>MNIIAILNHMGVYFKEEPIRELHKALEALDFQIVYPNDREDLLKLIDNNARLCGVIFDWDTYNLDLCEEISAMNEHLPVYAFANTHSTLDVSLNDLRLNVEFFEYALGAAQDIAQKIRQSTDAYIDEILPPLTKALFNYVKEGKYTFCTPGHMGGTAFQKSPVGSIFYDFFGANAMKSDISISVGELGSLLDHSGPHKEAEEYIARTFNAERSYMVTNGTSTANKIVGMYSAPAGSTVLIDRNCHKSLTHLMMMSDITPIYFRPTRNAYGILGGIPKSEFQHDTIAERVAQTPNATWPVHAVVTNSTYDGLLYNTDYIKEALDVKSIHFDSAWVPYTNFSPIYKGLCGMSGGRVEGKVIYETQSTHKLLAAFSQASMIHVKGDINEETFNEAYMMHTSTSPHYGIVASTETAAAMMKGNAGKRLINGSIERAIRFRKEIKRLNSESEGWFFDVWQPEGIDEAKCWPLDSKDNWHGFKDIDNDHMYLDPIKVTLLTPGMQKDGSMADTGIPASI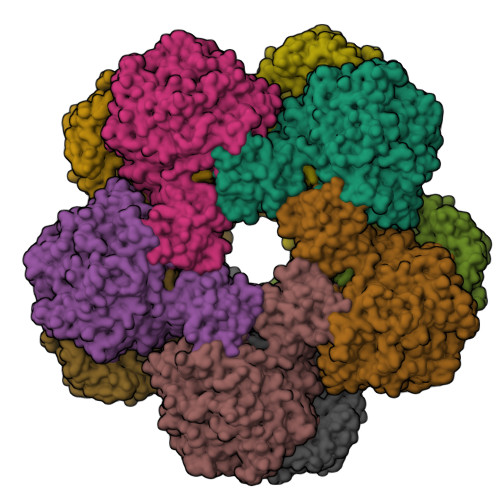VSKYLDEHGIIVEKTGPYNMLFLFSIGIDKTKALSLLRALTDFKRSYDLNLRVKNMLPSLYREDPEFYENMRIQELAQGIHALIQHHNLPDLMYRAFEVLPTMVMNPHAAFQMELRGQTEEVYLEEMIGKVNANMILPYPPGVPLVMPGEMLTEESRPVLEFLQMLCEIGAHYPGFETDIHGAYRQADGRYTVKVIK[10x]>KEENNFINLYTVKNPLKCKIVDKINLVRPNSPNEVYHLEINHNGLFKYLEGHTCGIIPYYNELDNNPNNQINKDHNIINTTNHTNHNNIALSHIKKQRCARLYSISSSNNMENLSVAIKIHKYEQTENAPNITNYGYCSGFIKNLKINDDIYLTGAHGYFNLPNDAIQKNTNFIFIATGTGISPYISFLKKLFAYDKNNLYNRNSNYTGYITIYYGVYNEDSILYLNELEYFQKMYPNNINIHYVFSYKQNSDATSFYVQDEIYKRKTEFLNLFNNYKCELYICGHKSIRYKVMDI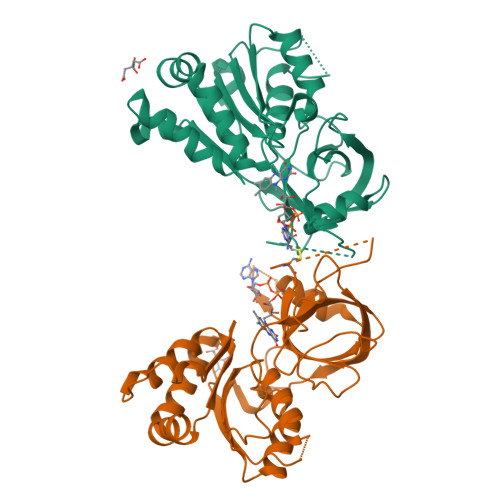LKSHDQFDEKKKKRVHVEVY[4x]>MSEILVLNCGSSSVKFALINPHTSQSLVTGLAENIATKNCKVVFKAEHKIVKYLENGSYKDVFEMLKDFLVENKHLEKIVAIGHRVVHGGQYFSKSVLINADSLEKIKACIALAPLHNPAHIEGIRFCQQIFPELPQVAVFDTAFHQTMPSYIAEYAIPYELTHKHNIRKYGAHGTSHKYVSEQAAKILTQQKANVIVAHLGNGCSITAVVDGKSIDTSMGLTPLDGLVMGTRSGCIDPSIFAYISDNLGWSVTEITNMLNKQSGLLGICGHNDMRE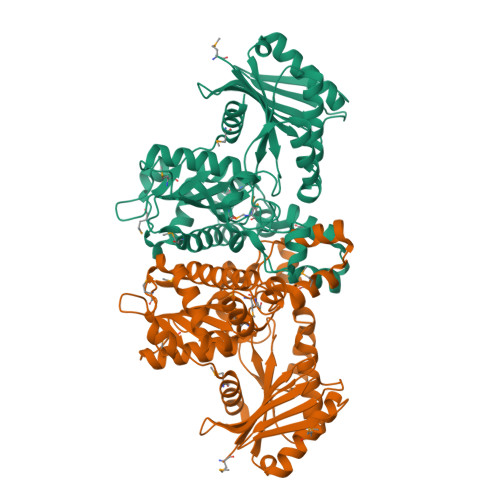VSQLAAKGDSLAKLAIEIFSHRVAKFVASYMIYFNKLDALVFTGGIGENAANIRKNIISKLANLGFMIDHQKNSNSETFINSKNSHNIMVIATNEELMIAQETQNLI[2x]3-(methylsulfanyl)propanoic acid | C4 H8 O2 S | 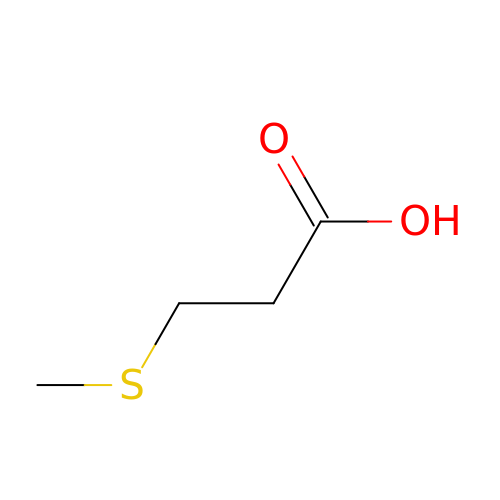CAOMCZAIALVUPA-UHFFFAOYSA-N>MVEGAVKTEPVDLFHPGFLNSSNYRIPALFKTKEGTLIASIDARRQGGADAPNNDIDTAVRRSEDGGKTWDEGQIIMDYPDKSSVIDTTLIQDDETGRIFLLVTHFPSKYGFWNAGLGSGFKNIDGKEYLCLYDSSGKEFTVRENVVYDKDGNKTEYTTNALGDLFRNGTKIDNINSSTAPLKAKGTSYINLVYSDDDGKTWSEPQNINFQVKKDWMKFLGIAPGRGIQIKNGEHKGRIVVPVYYTNEKGKQSSAVIYSDDSGKNWTIGESPNDNRKLENGKIINSKTLSDDAPQLTECQVVEMPNGQLKLFMRNLSGYLNIATSFDGGATWDETVEKDTNVLEPYCQLSVINYSQKIDGKDAVIFSNPNARSRSNGTVRIGLINQVGTYENGEPKYEFDWKYNKLVKPGYYAYSCLTELSNGNI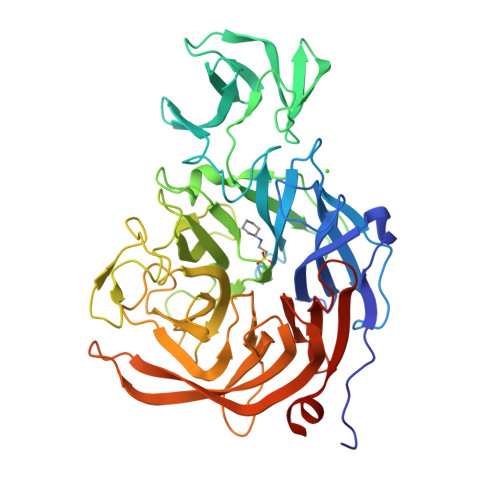GLLYEGTPSEEMSYIEMNLKYLESGANKLEHHHHHH[2x]>[2x]AECSVDIQGNDQMQ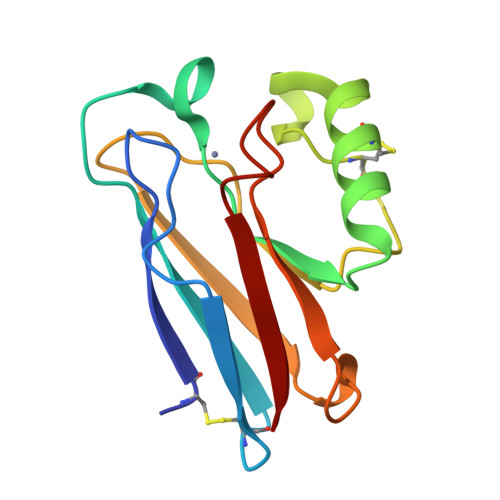FNTNAITVDKSCKQFTVNLSHPGNLPKNVMGHNWVLSTAADMQGVVTCGMASGLDKDYLCPDDSRVIAHTKLIGSGEKDSVTFDVSKLKEGEQYMFFCTFPGHSALMKGTLTLK> MTVRTRVTDLLEIEHPILMGGMAWAGTPTLAAAVSEAGGLGIIGSGAMKPDDLRKAISELRQKTDKPFGVNIILVSPWADDLVKVCIEEKVPVVTFGAGNPTKYIRELKENGTKVIPVVASDSLARMVERAGADAVIAEGMESGGHIGEVTTFVLVNKVSRSVNIPVIAAGGIADGRGMAAAFALGAEAVQMGTRFVASVESDVHPVYKEKIVKASIRDTVVTGAKLGHPARVLRTPFARKIQEMEFENPMQAEEMLVGSLRRAVVEGDLERGSFMVGQSAGLIDEIKPVKQIIEDILKEFKETV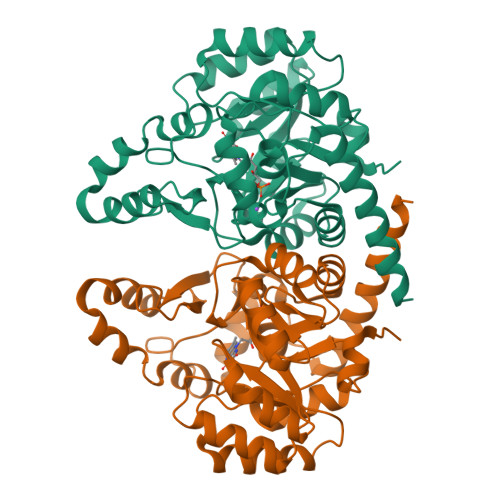EKLRGYIEE> MPAPHGGILQDLIARDALKKNELLSEAQSSDILVWNLTPRQLCDIELILNGGFSPLTGFLNENDY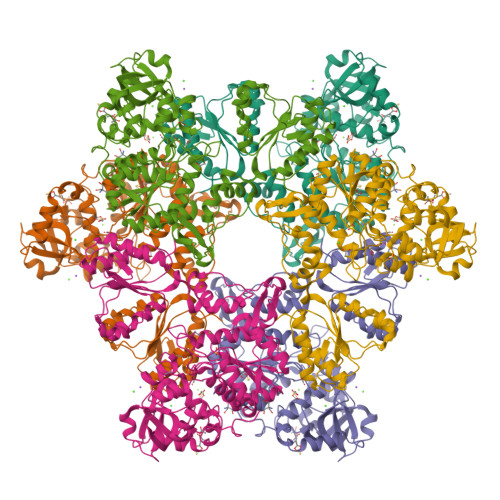SSVVTDSRLADGTLWTIPITLDVDEAFANQIKPDTRIALFQDDEIPIAILTVQDVYKPNKTIEAERVFRGDPEHPAISYLFNVAGDYYVGGSLEAIQLPQHYDYPGLRKTPAQLRLEFQSRQWDRVVAFQTRNPMHRAHRELTVRAAREANAKVLIHPVVGLTKPGDIDHHTRVRVYQEIIKRYPNGIAFLSLLPLAMRMSGDREAVWHAIIRKNYGASHFIVGRDHAGPGKNSKGVDFYGPYDAQELVESYKHELDIEVVPFRMVTYLPDEDRYAPIDQIDTTKTRTLNISGTELRRRLRVGGEIPEWFSYPEVVKILRESNPPRPKQGFSIVLGNSLTVSREQLSIALLSTFLQFGGGRYYKIFEHNNKTELLSLIQDFIGSGSGLIIPDQWEDDKDSVVGKQNVYLLDTSSSADIQLESADEPISHIVQKVVLFLEDNGFFVF> SMVKDWIPISHDNYKQVQGPFYHGTKANLAIGDLLTTGFISHFEDGRILKHIYFSALMEPAVWGAELAMSLS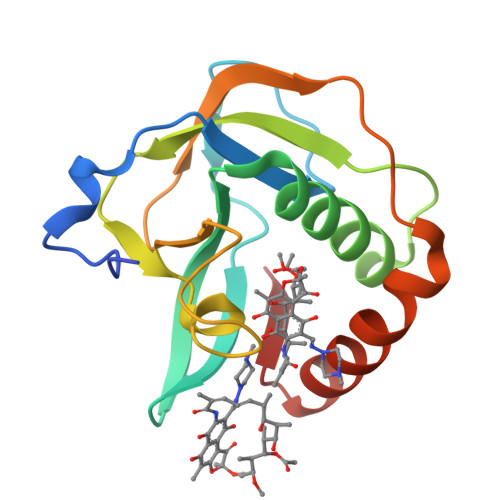GLEGRGYIYIVEPTGPFEDDPNLTNKKFPGNPTQSYRTCEPLRIVGVVEDWEGHPVELIRGMLDSLEDLKRRGLHVIED> QPSKDEGVLKEISITHHVKAGSEKADPSHFELLKVLGQGSFGKVFLVRKVTRPDSGHLYAMKVLKKATLKVRDRVRTKMERDILADVNHPFVVKLHYAFQTEGKLYLILDFLRGGDLFTRLSKEVMFTEEDVKFYLAELALGLDHLHSLGIIYRDLKPENILLDEEGHIKLTDFGLSKEAIDHEKKAYSFCGTVEYMAPEVVNRQGHSHSADWWSYGVLMFEMLTGSLPFQGKDRKETMTLILKAKLGMP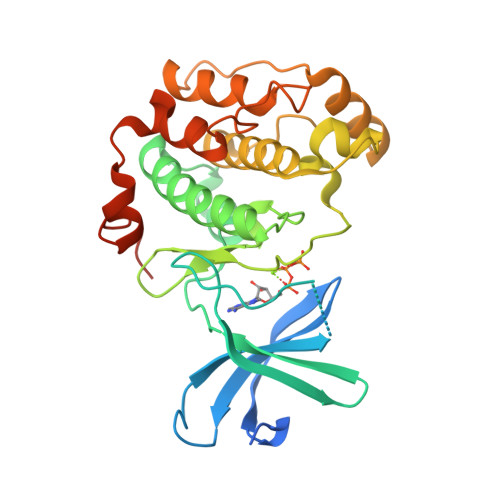QFLSTEAQSLLRALFKRNPANRLGSGPDGAEEIKRHVFYSTIDWNKLYRREIKPPFKPAVAQPDDTFYFDT methyl 1-(methanesulfonyl)-2-methyl-D-prolinate 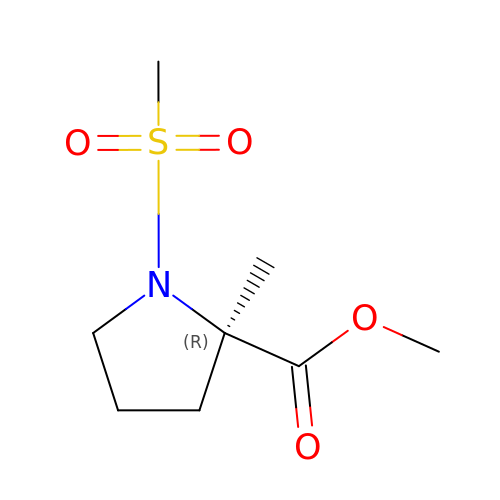| C8 H15 N O4 S | APDJGJFQSBOQHM-MRVPVSSYSA-N> MEFFGESWKKHLSGEFGKPYFIKLMGFVAEERKHYTVYPPPHQVFTWTQMCDIKDVKVVILGQDPYHGPNQAHGLCFSVQRPVPPPPSLENIYKELSTDIEDFVHPGHGDLSGWAKQGVLLLNAVLTVRAHQANSHKERGWEQFTDAVVSWLNQNSNGLVFLLWGSYAQKKGSAIDRKRHHVLQTAHPSPL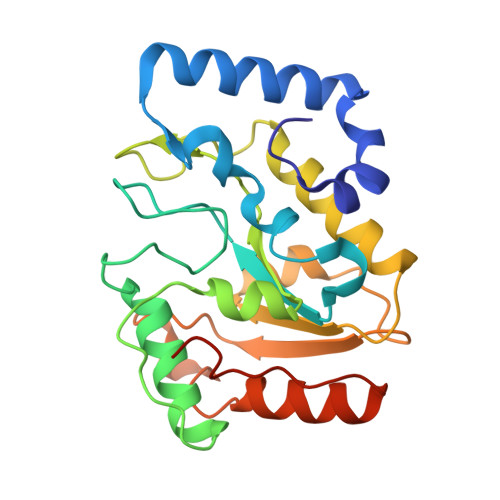SVYRGFFGCRHFSKTNELLQKSGKKPIDWKELLEHHHHHH>AEIYNKDGNKVDLYGKAVGLHYFSKGNGENSYGGNGDMTYARLGFKGETQINSDLTGYGQWEYNFQGNNSEGADAQTGNKTRHAFAGLKYADVGSFDYGRNHGVVYDALGYTDMLPEFGGDTAYSDDFFVGHVGGVATYRNSNFFGLVDGLNFAVQYLGKNERDTARRSNGDGVGGSISYEYEGFGIVGAYGAADRTNLQEAQPLGNGKKAEQWATGLKYDANNIYLAANYGETRNATPITNKFTNTSGFAN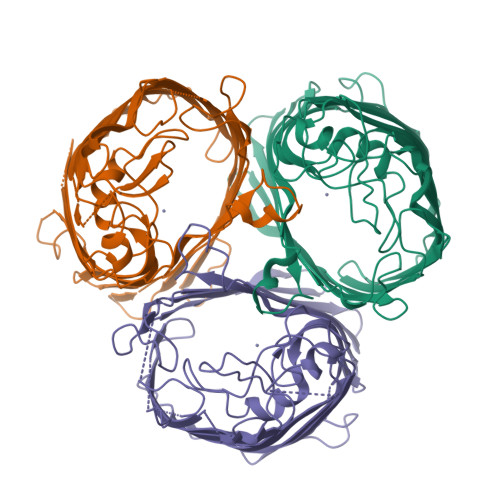KTQDVLLVAQYQFDFGLRPSIAYTKSKAKDVEGIGDVDLVNYFEVGATYYFNKNMSTYVDYIINQIDSDNKLGVGSDDTVAVGIVYQF[3x]> EVTDQLEDLREHFKNTEEGKALVHHYEECAERVKIQQQQPGYADLEHKEDCVEEFFHLQHYLDTATAPRL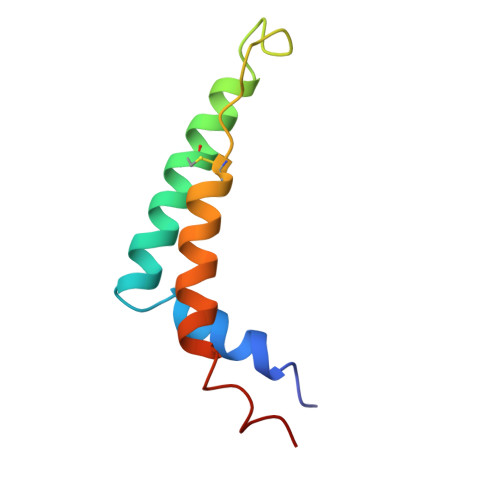FDKLK TRIHYDROGEN THIODIPHOSPHATE | H3 O6 P2 S | 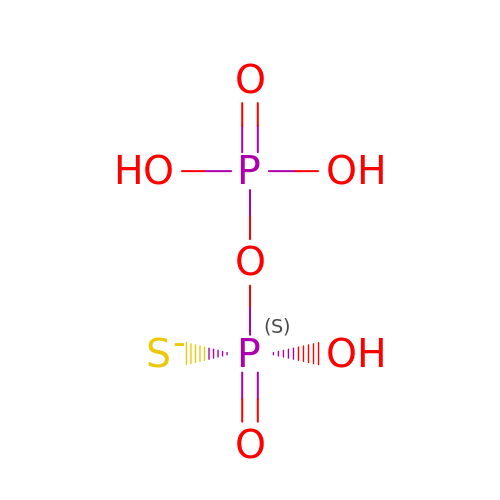HWTUHTNZLQJJEV-UHFFFAOYSA-M5'-O-(N-(L-seryl)-sulfamoyl)cytidine | C12 H19 N5 O9 S | 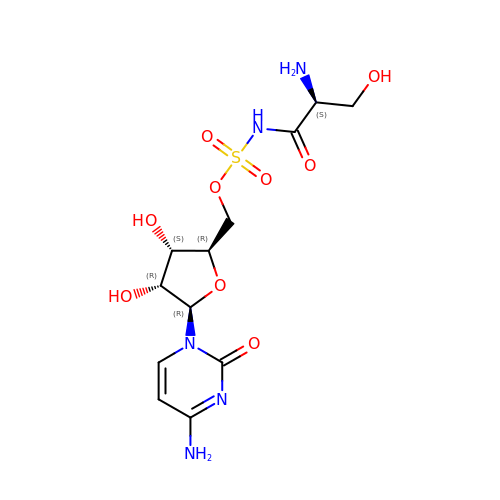KLHALWQAANSHJB-DANLAGSESA-N> MHHHHHHMGLNTAIATRVNGTPPPEVPIADIELGSLDFWALDDDVRDGAFATLRREAPISFWPTIELPGFVAGNGHWALTKYDDVFYASRHPDIFSSYPNITINDQTPELAEYFGSMIVLDDPRHQRLRSIVSRAFTPKVVARIEAAVRDRAHRLVSSMIANNPDRQADLVSELAGPLPLQIICDMMGIPKADHQRIFHWTNVILGFGDPDLATDFDEFMQVSADIGAYATALAEDRRVNHHDDLTSSLVEAEVDGERLSSREIASFFILLVVA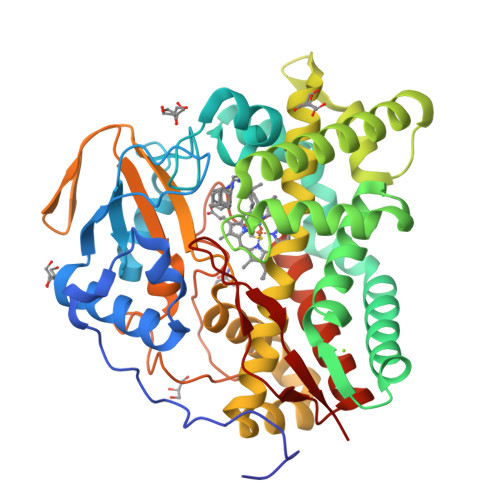GNETTRNAITHGVLALSRYPEQRDRWWSDFDGLAPTAVEEIVRWASPVVYMRRTLTQDIELRGTKMAAGDKVSLWYCSANRDESKFADPWTFDLARNPNPHLGFGGGGAHFCLGANLARREIRVAFDELRRQMPDVVATEEPARLLSQFIHGIKTLPVTWS> GKKN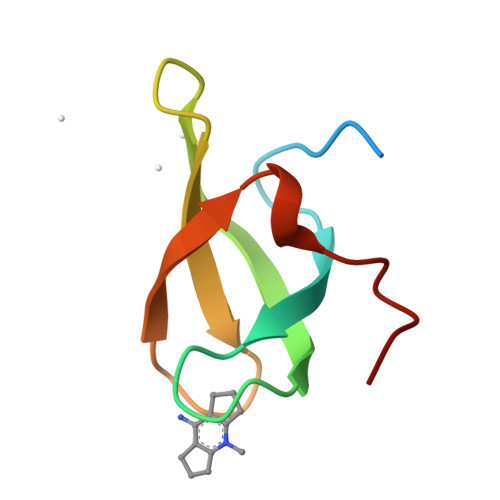TAASLQQWKVGDKCSAIWSEDGCIYPATIASIDFKRETCVVVYTGYGNREEQNLSDLLSPICE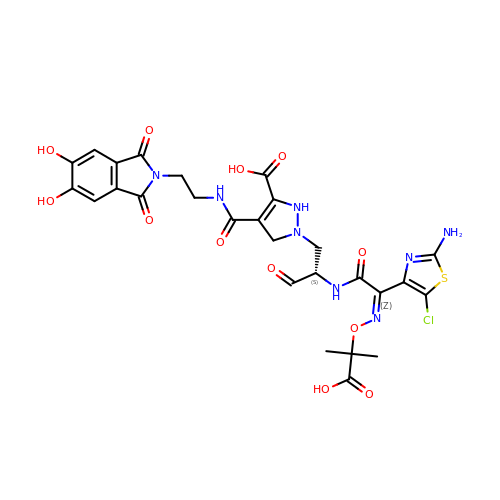1-[(2S)-2-{[(2Z)-2-(2-amino-5-chloro-1,3-thiazol-4-yl)-2-{[(2-carboxypropan-2-yl)oxy]imino}acetyl]amino}-3-oxopropyl]-4-{[2-(5,6-dihydroxy-1,3-dioxo-1,3-dihydro-2H-isoindol-2-yl)ethyl]carbamoyl}-2,5-dihydro-1H-pyrazole-3-carboxylic acid | C27 H27 Cl N8 O12 S | USNGVNQJWJJOSD-RUDQHFNBSA-N> SKMFFINDETPWEELGNGIKRKVMTWSDDLMMVCVHFDKGAIGVAHKHDIHDQIAYVAAGSFEVEIEGQKRILKAGDAYRAVKNEMHGAVSLEDNSILI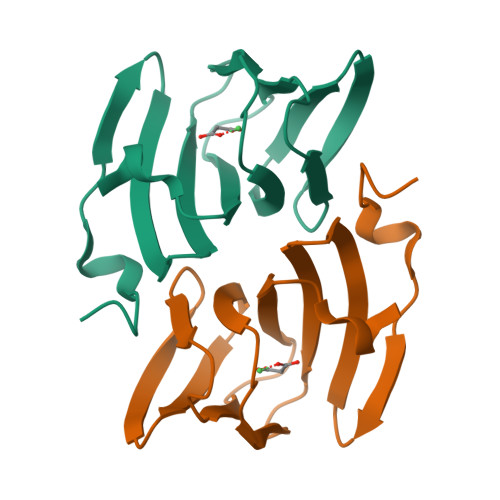DTFNPKRDDFL>[4x]MAHHHHH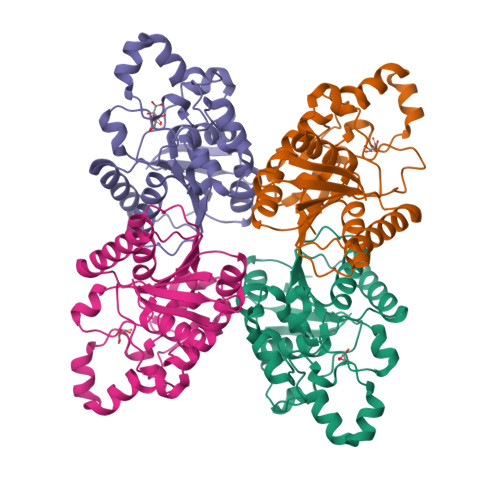HMELVFIRHGQSEWNAKNLFTGWRDVKLSEQGLAEAAAAGKKLKENGYEFDIAFTSVLTRAIKTCNIVLEESDQLFVPQIKTWRLNERHYGRLQGLDKKQTAEKYGDEQVRIWRRSYDTLPPLLDKDDAFSAHKDRRYAHLPADVVPDGENLKVTLERVLPFWEDQIAPAILSGKRVLVAAHGNSLRALAKHIEGISDEDIMGLEIPTGQPLVYKLDDNLKVIEKFYL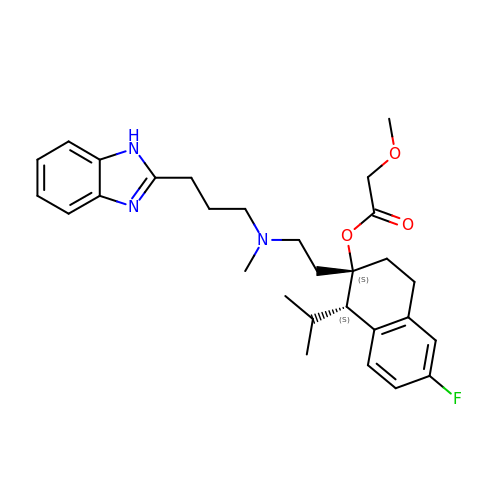(1S,2S)-2-(2-{[3-(1H-benzimidazol-2-yl)propyl](methyl)amino}ethyl)-6-fluoro-1-(propan-2-yl)-1,2,3,4-tetrahydronaphthalen-2-yl methoxyacetate | C29 H38 F N3 O3 | HBNPJJILLOYFJU-VMPREFPWSA-N> MNKRGLYSKLGISVVGISLLMGVPTLIHANELNYGQLSISPIFQGGSYQLNNKSIDISSLLLDKLSGESQTVVMKFKADKPNSLQALFGLSNSKAGFKNNYFSIFMRDSGEIGVEIRDAQKGINYLFSRPASLWGKHKGQAVENTLVFVSDSKDKTYTMYVNGIEVFSETVDTFLPISNINGIDKATLGAVNREGKEHYLAKGSIDEISLFNKAISDQEVSTIPLSNPFQLIFQSGDSTQANYFRIPTLYTLSSGRVLSSIDARYGGTHDSKSKINIATSYSDDNGKTWSEPIFAMKFNDYEEQLVYWPRDNKLKNSQISGS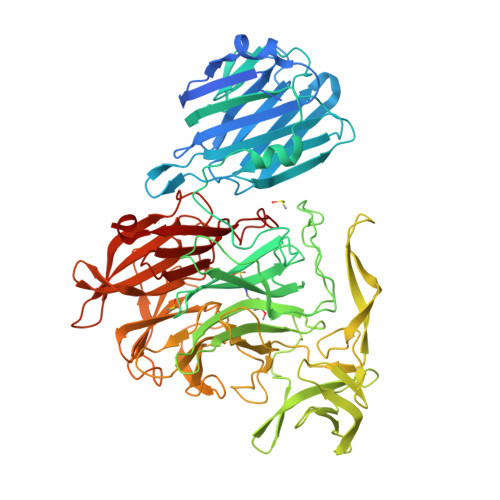ASFIDSSIVEDKKSGKTILLADVMPAGIGNNNANKADSGFKEINGHYYLKLKKNGDNDFRYTVRENGVVYNETTNKPTNYTINDKYEVLEGGKSLTVEQYSVDFDSGSLRERHNGKQVPMNVFYKDSLFKVTPTNYIAMTTSQNRGESWEQFKLLPPFLGEKHNGTYLCPGQGLALKSSNRLIFATYTSGELTYLISDDSGQTWKKSSASIPFKNATAEAQMVELRDGVIRTFFRTTTGKIAYMTSRDSGETWSKVSYIDGIQQTSYGTQVSAIKYSQLIDGKEAVILSTPNSRSGRKGGQLVVGLVNKEDDSIDWKYHYDIDLPSYGYAYSAITELPNHHIGVLFEKYDSWSRNELHLSNVVQYIDLEINDLTK> GSSRAMGNEVAGVEDISVEITPSSKRNSDARRTSRNCSSNEERKRRKYFHMLYLVCLMVHGFIRNEWINSKRLSRKLSNLVPEKVFELLHPQKDEELPLRSTRKLLDGLKKCMELWQKHWKITKKYDNEGLYMRTWKEIEMSANNKRKFKTLKRSDFLRAVSKGHGDPDISVQGFVAMLRACNVNARLIMSCQPPDFTNMKIDTSLNGNNAYKDMVKYPIFWCEVWDKFSKKWITVDPVNLKTIEQVRLHSKLAPKGVACCERNMLRYVIAYDRKYGCRDVTRRYAQWMNSKVRKRRITKDDFGEKWFRKVITALHHRKRTKIDDYEDQYFFRRDESEGIPDSVQDLKNHPYYVLEQDIKQTQIVKPGCKECGYLKVHGKVGKVLKVYAKRDIADLKSARQWYMNGRILKTGSRCKKVIKRTVGRPKGEAEEEDERLYSFEDTELYIPPLASASGEITKNTFGNIEVFAPTMIPGNCCLVENPVAIKAARFLGVEFAPAVTSFKFERGSTVKPVLSGIVVAKWLREAIETAIDGIEFI;> GSGNASSGALGTTGGATDAAQGGPPGSIGLTVEDLLSLRQVVSGNPEALAPLLENISARYPQLREHIMANPEVFVSMLLEAVGDNMQDVMEGADDMVEGEDIEVTGEAAAAGLGQGEGEGSFQVDYTPEDDQAISRLCELGFERDLVIQVYFACDKNEEAAANILFSDHAD

The mammalian global genome nucleotide excision repair (NER) factor, xeroderma pigmentosum C (XPC)–RAD23B complex (hereafter XPC), in particular, faces a difficult challenge. Once bound to a lesion, XPC recruits the multi-subunit transcription factor IIH (TFIIH) that verifies the lesion, which ultimately coordinates the assembly of NER factors, causing excision of a lesion-containing single-stranded DNA and repair synthesis that restores the duplex. The previous crystal structures of the yeast XPC orthologue, Rad4, bound to model lesions have shown that Rad4 and, by analogy, XPC recognize the damaged DNA site by inserting a β-hairpin into DNA duplex and flipping out damage-containing nucleotide pairs to form an ‘open’ conformation. In this conformation, Rad4 interacts exclusively with the two nucleotides on the undamaged strand without making specific contacts with the two damaged residues of the model UV lesion.

Here we present the first crystal structure in which Rad4 is captured on a single register of undamaged DNA using disulphide tethering. To overcome this problem, we covalently tethered Rad4 to undamaged DNA in a fixed register using a disulphide crosslinking method and solved a 3.05 Å structure of this complex. To our surprise, we found that this tethered complex formed an ‘open’ conformation that is essentially indistinguishable from the lesion-bound structure8. Note that the disulphide tethering was made at a position distant from the flipped-out nucleotides and, therefore, it is unlikely that the ‘open’ conformation was due to structural perturbations from crosslinking. The overall root mean squared deviation between this complex and the lesion-bound complex structures is 0.99 Å for 2,388 main-chain atoms including both protein and DNA. In this Rad4–undamaged DNA structure, the DNA is bent by ~42° as in the lesion-bound structure. Our structure shows that tethered Rad4 flips out normal nucleotide pairs and forms the same ‘open’ conformation as with damaged DNA. These results indicate that structural discrimination between normal and damaged DNA cannot be the basis for lesion recognition by Rad4/XPC, and instead points to a novel ‘kinetic gating’ mechanism, whereby the DNA lesion selectivity arises mainly from the kinetic competition between Rad4-induced DNA opening and the residence time of Rad4 at a given site. In our structural study, chemical tethering of Rad4 on DNA prolonged Rad4’s residence time indefinitely, thus allowing even undamaged DNA to be fully opened. To our knowledge, the presented crystal structure is the first high-resolution structure of a nonspecific DNA-bound, DNA repair protein that relies exclusively on indirect read-out and makes no direct contacts with the damaged nucleotides in the specific recognition complex.>ETFDGLAPYVETFNNRGCEFPKSGYEGPASNDDNDEMCVKVSMLRVKVSQSYAAKQIQQFSGFKESGIDVKQISNVKKIY[2x];>MLDAFSKVITSADGKAAYVGGADLQALKKFVSEGNKRMDSVNAIVSNASCIVSDSVSGMVCENPSLIAPNGGVYTNRKMAACLRDAEIILRYVSYSLLSGDSSVLEDRCLNGLKETYASLGVPAAGNARTISIMKATVIGFITNNSQQKKLSTPAGDCSALASEVGGYFDKVSSALA[4x];>KTDNKLRAPIITVFDARGCREHKNREYKGPKTGTQDDEMCVKVQYEKIAACEDTAFIVLKECLSEMKS[2x]

Cryptophyte algae have a unique phycobiliprotein light-harvesting antenna that fills a spectral gap in chlorophyll absorption from photosystems. We show that the cryptophyte Hemiselmis andersenii expresses an energetically complex antenna comprising three distinct spectrotypes of phycobiliprotein, each composed of two αβ protomers but with different quaternary structures arising from a diverse α subunit family. We report crystal structures of the major phycobiliprotein from each spectrotype. We propose that the macromolecular organization of the cryptophyte antenna consists of bulk open and open-braced forms that transfer excitations to photosystems via this bridging closed form phycobiliprotein.

The final components (~15%) are closed forms with a long wavelength spectral feature due to substitution of a single chromophore. This chromophore is present on only one β subunit where asymmetry is dictated by the corresponding α subunit. The structure of the closed form HaPE645 provides an explanation for its unusual spectral properties. Our electron density maps clearly demonstrate that the chromophore attached to Cys82 on the β subunit in the αSβ protomer is unambiguously PCB (which causes the secondary absorption peak for this protein at 645 nm), while the chromophore attached to Cys82 on the β subunit in the αLβ protomer is unambiguously PEB. The N-terminal region of the α subunit appears to dictate the chemical nature of the chromophore attached to Cys82 on the associated β subunit. In each αβ protomer, the N-terminal tail of the respective α subunit interacts with pyrrole ring D of the β82 chromophore. For the αSβ protomer, the side chain of Leu6 packs against the face of pyrrole ring D of PCB β82. This pocket is specific for PCB and incompatible with a PEB chromophore due to the steric clash that would be created by Leu6 (Fig. 3d compared to Fig. 3f). The excitation-emission map for HaPE645 suggests that this protein acts as an energy adaptor with excitation transfer from higher energy (562 nm) to lower energy (650 nm) chromophores within the protein. The spectral properties of HaPE645, a much smaller constituent fraction of the cryptophyte PBP antenna (~1/7 of the PBPs), fulfil the requirements for a terminal acceptor of the soluble PBP antenna that acts as the adaptor to bridge the energy gap and transfer the excitations to the integral membrane photosystems embedded in the thylakoid membrane which have a local absorption maximum at 668 ± 3 nm (e green spectrum).> XGAQVSSQKVGAHENSSTINYTTINYYRDSASNA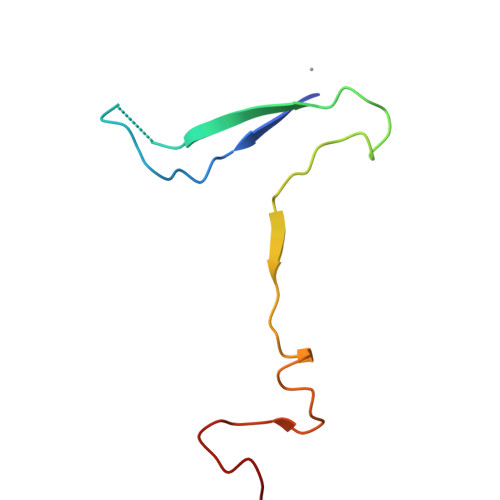ASKQDFSQDPSKFTEPIKDVLIKTAPMLN>PP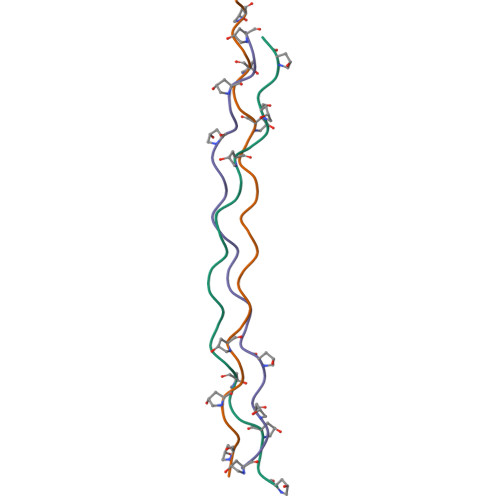GPPGPPGEKGDRGFPGPPGPPGPPG[6x]>MASRAPKEVPLCPLMTDGETRNVTDLPGPTNWPLLGSLLEIFWKGGLKKQHDTLAEYHKKYGQIFRMKLGSFDSVHLGSPSLLEALYRTESAHPQRLEIKPWKAYRDHRNEAYGLMILEGQEWQRVRSAFQKKLMKPVEIMKLDKKINEVLADFLERMDELCDERGRIPDLYSELNKWSFESICLVLYEKRFGLLQKETEEEALTFITAIKTMMSTFGKMMVTPVELHKRLNTKVWQAHTLAWDTIFKSVKPCIDNRLQRYSQQPGADFLCDIYQQDHLSKKELYAAVTELQLAAVETTANSLM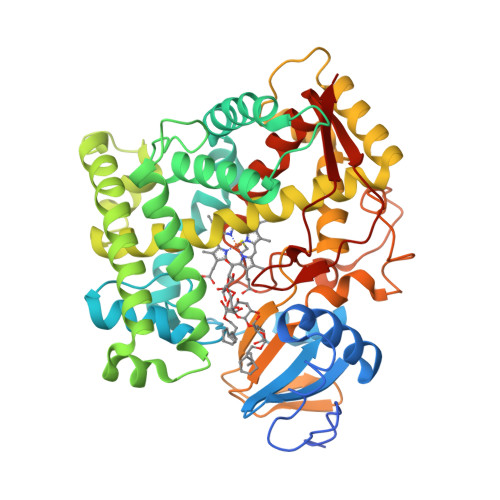WILYNLSRNPQAQRRLLQEVQSVLPDNQTPRAEDLRNMPYLKACLKESMRLTPSVPFTTRTLDKPTVLGEYALPKGTVLTLNTQVLGSSEDNFEDSHKFRPERWLQKEKKINPFAHLPFGIGKRMCIGRRLAELQLHLALCWIIQKYDIVATDNEPVEMLHLGILVPSRELPIAFRPR[2x]> MGSDTETTDSTKFTIYYTGMTDIGPSMTGVISSPTYKGGTPYDFAITRITLDGEPFSDSIFAIDSETGKITLNSTSNTPVGLYKLSVACYSNNNRYEYTDIVEINMMKPVPDGIKTDPEKLQVEYADIIDTESSNELPTSQIRTEGNHISISNYTIASAMWNGVAVESPEDYFAVSDKGEISIIKGNQNIQPGKYILSFKLTTAATGEDPEKGIFENALEINVTSRPLSLIYTPDEGKIEEEGERSPETTFQSNIPALKGSAEGLVYSISSVSPNTDKITIDPTTGVLSVAAHHGFKDGEKYQISVKAINEFSPEGVVFENVFTLNTVEFIEPIANFGYADVNDVQAVEIDINKNENFKGDEVKYEFVNLPTDLQGELALDLDGNIAIKKGNKIPVGQYTVQVMATNTK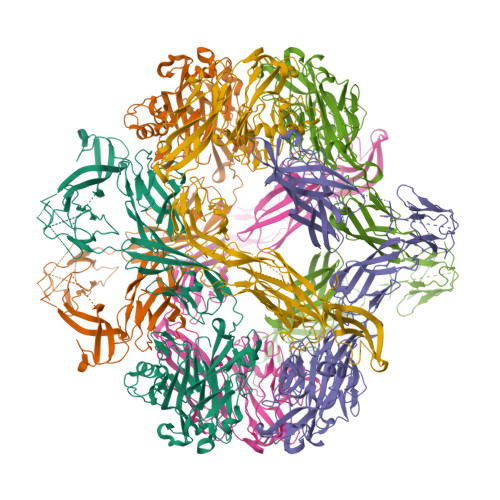GSETATFTLTITANPNYFTYFRYGNNLGLTPIENYADQFRIEAGGKLNSVKPVPTATDAKDGLSSLKWEVELKHNPNNTKATINESTGQITITGLKQGQCGMVMVTATAGEGKTAVSVKQPVFFHFSMISDSNVQLEYTPFVFQVNPARGGESIAPSLGAGIDKSTFRLDYRRDFFYYNIAGPDSHISGALAQKVDNFLSEMWNSYDATAGTSRKPMSYFENTTNLSKALGYIDQTDFKVHINPNLWRNKDGYANGAMIGQITYDVTGKDPQAATSGARVSPIFIWFDTKFLEHHHHHH6-HYDROXYMETHYLPTERIN-DIPHOSPHATE | C7 H9 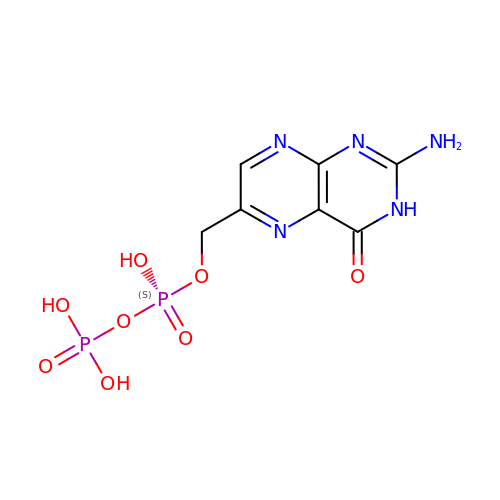N5 O8 P2 | AMDUVUKDRBIVAH-UHFFFAOYSA-N>[10x]GANAMASMKFAVIDRKNFTLIHFEIEKPIKPEILKEIEIPSVDTRKGVVISGRGPIWLHCFLAHKYAHTPFVAVYDPRLGAVVVQSHSELREGDVIDVVVEEILKGGVRHV

Here, we focus on the Csx3 family of proteins, which is found associated with many type III CRISPR systems. We demonstrate that Csx3 is, in fact, a cA4-specific ring nuclease, for which we propose the name Crn3 (CRISPR-associated ring nuclease 3). The enzyme has an unusual cooperative reaction mechanism involving the association of two dimers, bridged by the cA4 substrate, to complete the active site. While we confirmed the main experimental observations of the original study, our analyses have revealed that Csx3 binds much more tightly to cA4 than to RNA, is considerably more active as a cA4-specific ring nuclease than an RNA deadenylase, and has properties consistent with a function as a ring nuclease in vivo. These data indicate that Csx3 functions as a cA4-specific ring nuclease in type III CRISPR systems.

In parallel with the biochemical analysis, we crystallised the H60A variant of Csx3 and soaked the cA4 substrate into the crystals. The structure was solved using molecular replacement with data to 1.84 Å resolution. The electron density clearly showed a molecule of cA4 bound between adjacent dimers of Csx3. Notably, the Csx3 structure presented here crystallised in a different space group to those structures published previously, which has allowed the arrangement of Csx3 dimers into a pseudo filament arrangement with a cA4 molecule sandwiched between the D69 and H60 faces of the protein. The rotation between adjacent dimers in the filament is 144 °, coupled with a translation of 28 Å. The majority of interactions are made by the D69 face. The cA4 hydrogen bonds with the main chain atoms of I22, S44, G45, and I49, and side chain atoms of S44, R46 and R71. The one interaction evident from the H60 face with cA4 is a strong (2.4–2.5 Å) hydrogen bond between H80 and the 2’-OH of the ribose ring. Interestingly, R71 moves around 3.3 Å in order to form bidentate hydrogen bonds with an oxygen atom of a phosphate group, which we predict is adjacent to the phosphodiester bond that is cleaved. We see no evidence for the ion in our crystal structure, which may be due to the deletion of the H60 side chain.>MKHQHQHQHQHQHQQPLNEEFRPEMLQGKKVIVTGASKGIGREMAYHLAKMGAHVVVTAR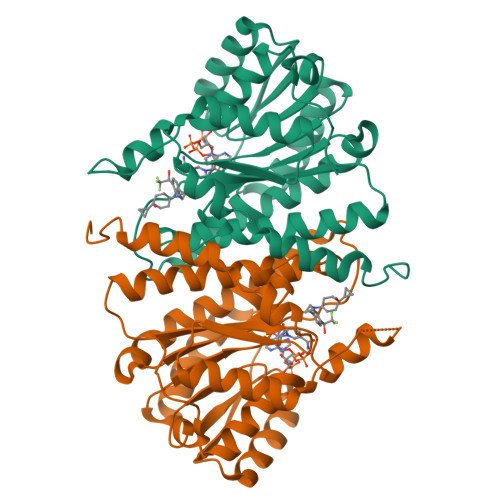SKETLQKVVSHCLELGAASAHYIAGTMEDMTFAEQFVAQAGKLMGGLDMLILNHITNTSLNLFHDDIHHVRKSMEVNFLSYVVLTVAALPMLKQSNGSIVVVSSLAGKVAYPMVAAYSASKFALDGFFSSIRKEYSVSRVNVSITLCVLGLIDTETAMKAVSGIVHMQAAPKEECALEIIKGGALRQEEVYYDSSLWTTLLIRNPSRKILEFLYSTSYNMDRFINK[2x]>[2x]MVGNYQGKKAIVIGGTHGMGLATVRRLVEGGAEVLLTGRNESNIARIREEFGPRVHALRSDIADLNEIAVLGAAAGQTLGAIDLLHINAGVSELEPFDQVSEASYDRQFAVNTKGAFFTVQRLTPLIREGGSIVFTSSVADEGGHPGMSVYSASKAAL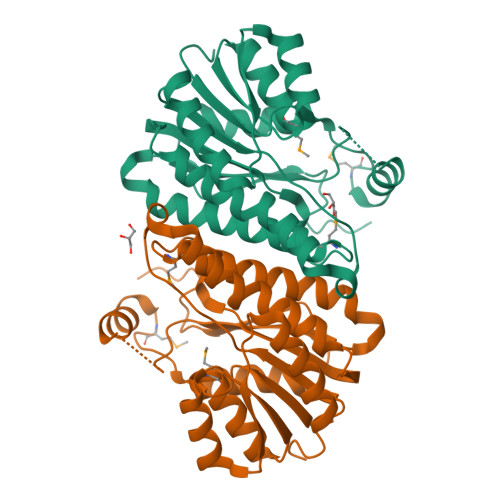VSFASVLAAELLPRGIRVNSVSPGFIDTPTKGVAGITEAERAEFKTLGDNITPMKRNGTADEVARAVLFLAFEATFTTGAKLAVDGGLGQKLSTAA> APA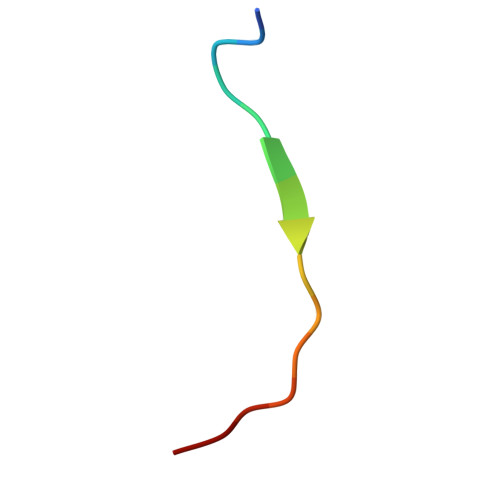TGGVMKPHRYRP7-[(3-aminopropyl)amino]heptane-2,2-diol | C10 H24 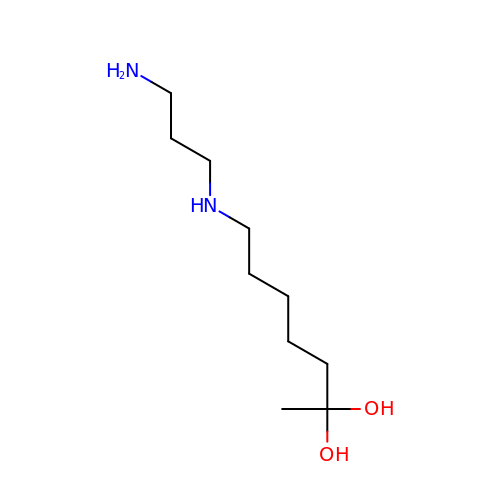N2 O2 | VZPARMKCSXRGQB-UHFFFAOYSA-N> MSLRIGVIGTGAIGKEHINRITNKLSGAEIVAVTDVNQEAAQKVVEQYQLNATVYPNDDSLLADENVDAVLVTSWGPAHESSVLKAIKAQKYVFCEKPLATTAEGCMRIVEEEIKVGKRLVQVGFMRRYDSGYVQLKEALDNHVIGEPLMIHCAHRNPTVGDNYTTDMAVVDTLVHEIDVLHWLVNDDYESVQVIYPKKSKNALPHLKDPQIVVIETKGGIVINAEIYVNCKYGYDIQCEIVGEDGIIKLPEPSSISLRKEGRFSTDILMDWQRRFVAAYDVEIQDFIDSIQKKGEVSGPTAWDGYIAAVTTDACVKAQESGQKEKVELKE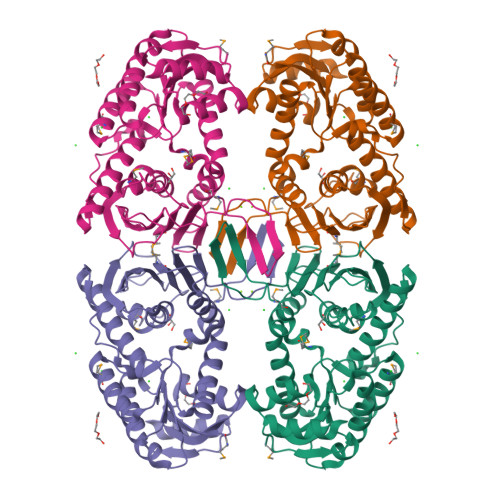KPEFYQSFTTVQN> MKILVAVKQTAALEEDFEIREDGMDVDEDFMMYDLNEWDDFSLEEAMKIKESSDTDVEVVVVSVGPDRVDESLRKCLAKGADRAVR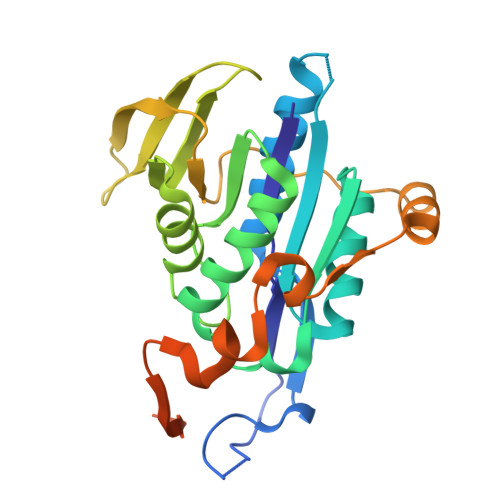VWDDAAEGSDAIVVGRILTEVIKKEAPDMVFAGVQSSDQAYASTGISVASYLNWPHAAVVADLQYKPGDNKAVIRRELEGGMLQEVEINCPAVLTIQLGINKPRYASLRGIKQAATKPIEEVSLADIGLSANDVGAAQSMSRVRRMYIPEKGRATMIEGTISEQAAKIIQIINEFKGA> MEELDGEPTVTLIPGVNSKKNQMYFDWGPGEMLVCETSFNKKEKSEMVPSCPFIYIIRKDVDVYSQILRKLFNESHGIFLGLQRIDEELTGKSRKSQLVRVSKNYRSVIRACMEEMHQVAIAAKDPANGRQFSSQVSILSAMELIWNLCEILFIEVAPAGPLLLHLLDWVRLHVCEVDSLSADVLGSENPSKHDSFWNLVTILVLQGRLDEARQMLSKEADASPASAGICRIMGDLMRTMPILSPGNTQTLTELELKWQHWHEECERYLQDSTFATSPHLESLLKIMLGDEAALLEQKELLSNWYHFLVTRLLYSNPTVKPIDLHYYAQSSLDLFLGGESSPEPLDNILLAAFEFDIHQVIKECSIALSNWWFVAHLTDLLDHCKLLQSHNLYFGSNMREFLLLEYASGLFAHPSLWQLG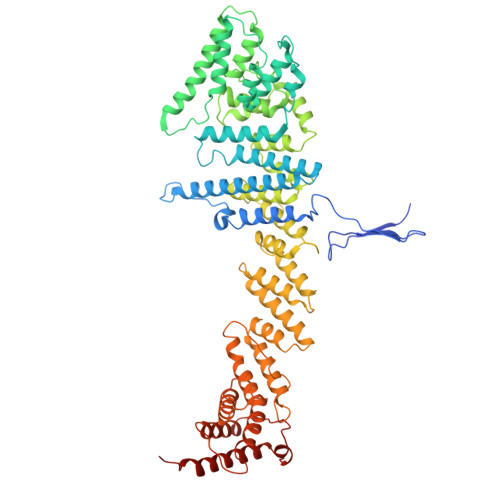VDYFDYCPELGRVSLELHIERIPLNTEQKALKVLRICEQRQMTEQVRSICKILAMKAVRNNRLGSALSWSIRAKDAAFATLVSDRFLRDYCERGCFSDLDLIDNLGPAMMLSDRLTFLGKYREFHRMYGEKRFADAASLLLSLMTSRIAPRSFWMTLLTDALPLLEQKQVIFSAEQTYELMRCLEDLTSRRPVHGESDTEQLQDDDIETTKVEMLRLSLARNLARAIIREGSLEGS> MRDTRFPCLCGIAASTLLFATTPAIAGEAPADRLKALVDAAVQPVMKANDIPGLAVAISLKGEPHYFSYGLASKEDGRRVTPETLFEIGSVSKTFTATLAGYALAQDKMRLDDRASQHWPALQGSRFDGISLLDLATYTAGGLPLQFPDSVQKDQAQIRDYYRQ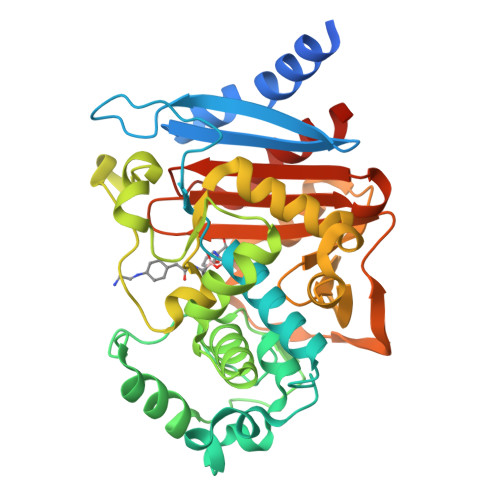WQPTYAPGSQRLYSNPSIGLFGYLAARSLGQPFERLMEQQVFPALGLEQTHLDVPEAALAQYAQGYGKDDRPLRVGPGPLDAEGYGVKTSAADLLRFVDANLHPERLDRPWAQALDATHRGYYKVGDMTQGLGWEAYDWPISLKRLQAGNSTPMALQPHRIARLPAPQALEGQRLLNKTGSTNGFGAYVAFVPGRDLGLVILANRNYPNAERVKIAYAILSGLEQQGKVPLKR>MEEPEEPADSGQSLVPVYIYSPEYVSMCDSLAKIPKRASMVHSLIEAYALHKQMRIVKPKVASMEEMATFHTDAYLQHLQKVSQEGDDDHPDSIEYGLGYDCPATEGIFDYAAAIGGATITAAQCLIDGMCKVAINWSGGWHHAKKDEASGFCYLNDAVLGILRLRRKFERILYVDLDLHHGDGVEDAFSFTSKVMTVSLHKFSPGFFPGTGDVSDVGLGKGRYYSVNVPIQDGIQDEKYYQICESVLKEVYQAFNPKAVVLQLGADTIAGDPMCSFNMTPVGIGKCLKYILQWQLATLILGGGGYNLANTARCWTYLTRVILGKTLSSEIPDH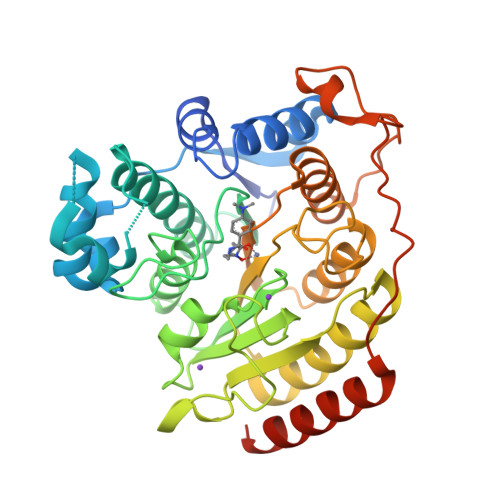EFFTAYGPDYVLEITPSCRPDRNEPHRIQQILNYIKGNLKHVVIEGRGSHHHHHH[2x]> MPKHGKRYRALLEKVDPNKIYTIDEAAHLVKELATAKFDETVEVHAKLGIDPRRSDQNVRGTVSLPHGLGKQVRVLAIAKGEKIKEAEEAGADYVGGEEIIQKILDGWMDFDAVVATPDVMGAVGSKLGRILGPRGLLPNPKAGTVGFNIGE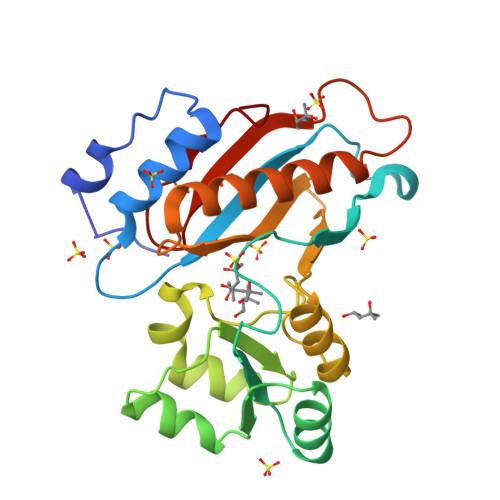IIREIKAGRIEFRNDKTGAIHAPVGKASFPPEKLADNIRAFIRALEAHKPEGAKGTFLRSVYVTTAMGPSVRINPHS>MTAVSEFRPGLEGVPATLSSISFVDGQRGVLEYRGISIEQLAQQSSFLETAYLLIWGHLPTQQELTEFEHEIRYHRRIKFRIRDMMKCFPDSGHPMDALQASAAALGLFYSRRALDDPEYIRAAVVRLLAKIPTMVAAFQLIRKGNDPIQPRDELDYAANFLYMLTEREPDPVAARIFDICLTLHAEHTINASTFSAMVTASTLTDPYAVVASAVGTLAGPLHGGANEEVLDMLEAIGSVENVEPYLDHCIATKTRIMGFGHRVYKVKDPRAVILQNLAE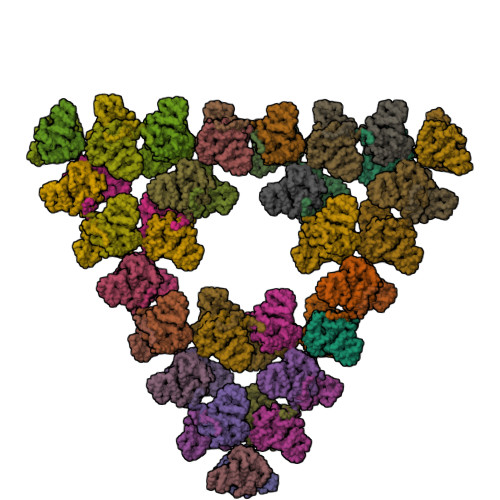QLFDIFGHDPYYEIAVAVEKAAAERLSHKGIYPNVDFYSGLVYRKLGIPSDLFTPVFAIARVAGWLAHWKEQLNENRIFRPTQIYTGSRNLDYTPIADRDLAIESDLEHHHHHH[54x]> MAEEHHHHHHHHLEVLFQGPPPGPRSPQREPQRVSHEQFRAALQLVVDPGDPRSYLDNFIKIGEGSTGIVCIATVRSSGKLVAVKKMDLRKQQRRELLFNEVVIMRDYQHENVVEMYNSYLVGDELWVVMEFLEGGALTDIVTHTRMNEEQIAAVCLAVLQALSVLHAQGVI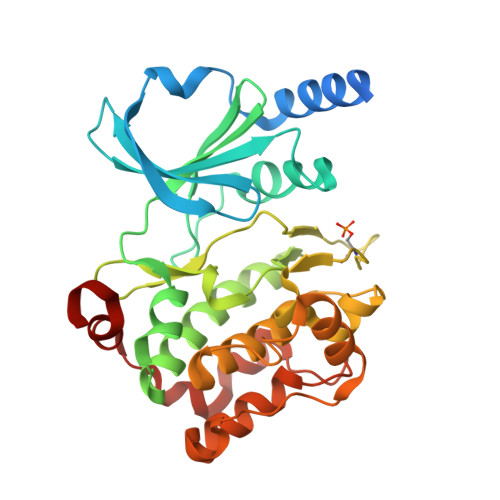HRDIKSDSILLTHDGRVKLSDFGFCAQVSKEVPRRKSLVGTPYWMAPELISRLPYGPEVDIWSLGIMVIEMVDGEPPYFNEPPLKAMKMIRDNLPPRLKNLHKVSPSLKGFLDRLLVRDPAQRATAAELLKHPFLAKAGPPASIVPLMRQNRTR> SNIGMILKERQDGVLVLTLNRPEKLNAITGELLDALYAALKEGEEDREVRALLLTGAGRAFSAGQDLTEFGDRKPDYEAHLRRYNRVVEALSGLEKPLVVAVNGVAAGAGMSLALWGDLRLAAVGASFTTAFVRIGLVPDSGLSFLLPRLVGLAKAQELLLLSPRLSAEEALALGLVHRVVPAEKLMEEALS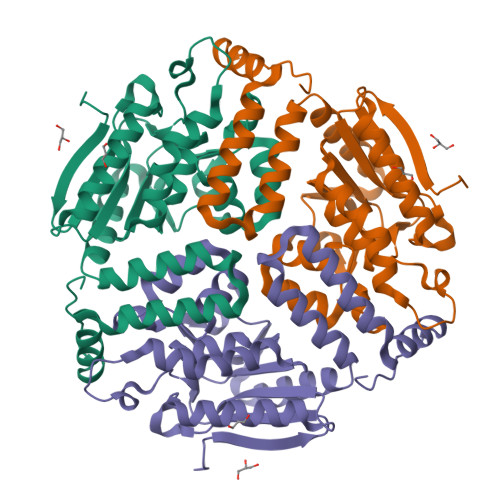LAKELAQGPTRAYALTKKLLLETYRLSLTEALALEAVLQGQAGQTQDHEEGVRAFREKRPPRFQGR>[8x]MDKFRVQGPTRLQGEVTISGAKNAALPILFAALLAEEPVEIQNVPKLKDIDTTMKLLTQLGTKVERDGSVWI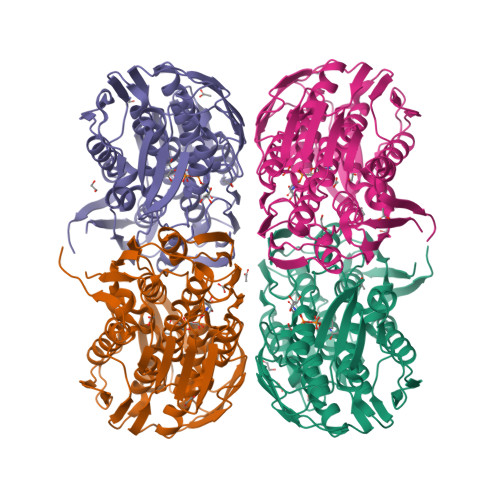DASNVNNFSAPYDLVKTMRASIWALGPLVARFGQGQVSLPGGDAIGARPVDLHIFGLEKLGAEIKLEEGYVKASVNGRLKGAHIVMDKVSVGATVTIMSAATLAEGTTIIENAAREPEIVDTANFLVALGAKISGQGTDRITIEGVERLGGGVYRVLPDRIETGTFLVAAAISGGKIVCRNAQPDTLDAVLAKLREAGADIETGEDWISLDMHGKRPKAVTVRTAPHPAFPTDMQAQFTLLNLVAEGTGVITETIFENRFMHVPELIRMGAHAEIESNTVICHGVEKLSGAQVMATDLRASASLVLAGCIAEGTTVVDRIYHIDRGYERIEDKLRALGANIERVKGE> AVVQRVEIHKLRQGENLILGFSIGGGIDQDPSQNPFSEDKTDKGIYVTRVSEGGPAEIAGLQIGDKIMQVNGWDMTMVTHDQARK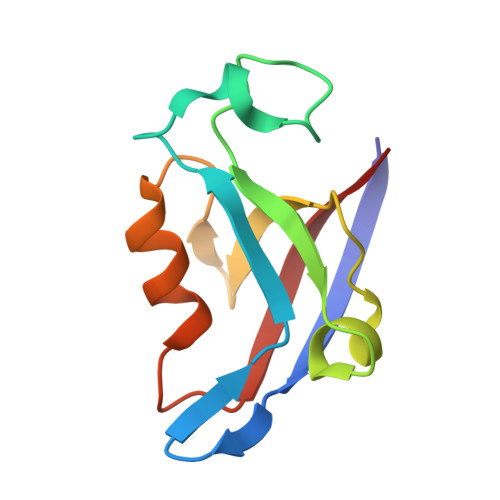RLTKRSEEVVRLLVTRQ> SHMGTRDDEYDYLFKVVLIGDSGVGKSNLLSRFTRNEFNLESKSTIGVEFATRSIQVDGKTIKAQIW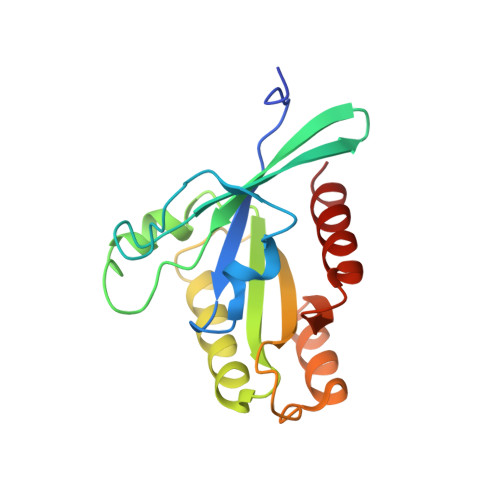DTAGQERYRAITSAYYRGAVGALLVYDIAKHLTYENVERWLKELRDHADSNIVIMLVGNKSDLRHLRAVPTDEARAFAEKNGLSFIETSALDSTNVEAAFQTILTEIY>GPGSCPTHADSLNNLANIKREQGNIEEAVRLYRKALEVFPEFAAAHSNLASVLQQQGKLQEALMHYKEAIRISPTFADAYSNMGNTLKEMQDVQGALQCYTRAIQINPAFADAHSNLASIHKDSGNIPEAIASYRTALKLKPDFPDAYCNLAHCLQIVCDWTDYDERMKKLVSIVADQLEKNRLPSVHPHHSMLYPLSHGFRKAIAERHGNLCLDKINVLHKPPYEHPKDLKLSDGRLRVGYVSSDFGNHPTSHLMQSIPGMHNPDKFEVFCYALSPDDGTNFRVKVMAEANHFIDLSQIPCNGKAADRIHQDGIHILVNMNGYTKGARNELFALRPAPIQAMWLGYPGTSGALFMDYIITDQETSPAEVAEQYSEKLAYMPHTFFIGDHANMFPHLKKKAVIDFKSNGHIYDNRIVLNGIDLKAFLDSLPDVKIVKMKCPDGGDNADSSNTALNMPVIPMNTIAEAVIEMINRGQIQITINGFSISNGLATTQINNKAATGEEVPRTIIVTTRSQYGLPEDAIVYCNFNQLYKIDPSTLQMWANILKRVPNSVLWLLRFPAVGEPNIQ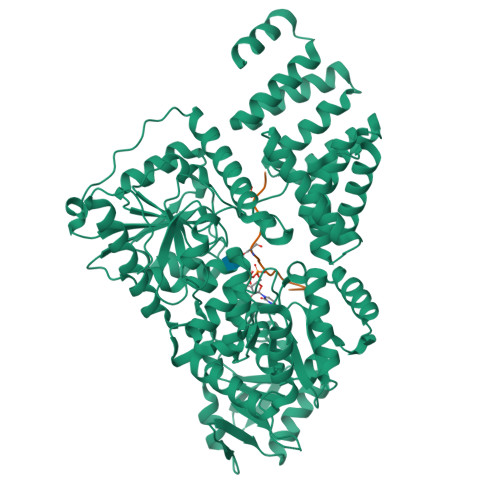QYAQNMGLPQNRIIFSPVAPKEEHVRRGQLADVCLDTPLCNGHTTGMDVLWAGTPMVTMPGETLASRVAASQLTCLGCLELIAKNRQEYEDIAVKLGTDLEYLKKVRGKVWKQRISSPLFNTKQYTMELERLYLQMWEHYAAGNKPDHMIKPVE[2x];>YPGGSTPVSSANMM[2x]> SNAMEETEAVQQDIEALEREIQTIKIQIANAHSGASKDEVKIPDAYKQFLSENINFSNLMRKDENTTLSINLSPRKPGTTTGQIQGIDSSIRSNFGVSSGHNEVAGFKSITDFVQWENSVRLIGVSLFPVNYDNIEFMGIRLELFDELSLKYDPPFYVILKPSVKRLGIWELFKHNLPKYINIHQHWQLITKDTDTSDSNIM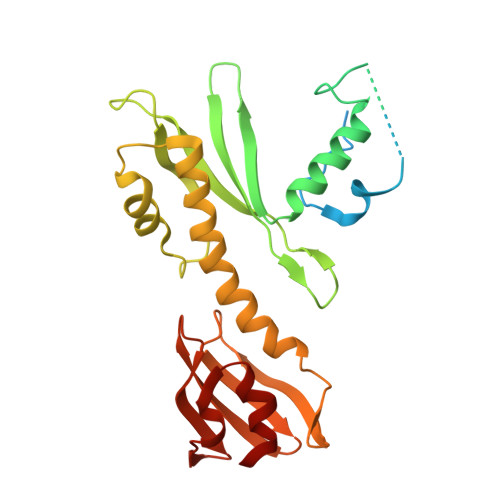KFANLCYKDLLKVHSRVQFFRKLEGNYVNDKQYSLLHIDNMGLNVSFRLGADIIKIKVDDGDDEIIDCTFNGEKNISLLGSIYGITNRFQSIIM>HMLEMIKSGKARAHTNIALIKYWGKKDEALIIPMNNSISVTLEKFYTETKVTFNDQLTQDQFWLNGEKVSGKELEKISKYMDIVRNRAGIDWYAEIESDNFVPTAAGLA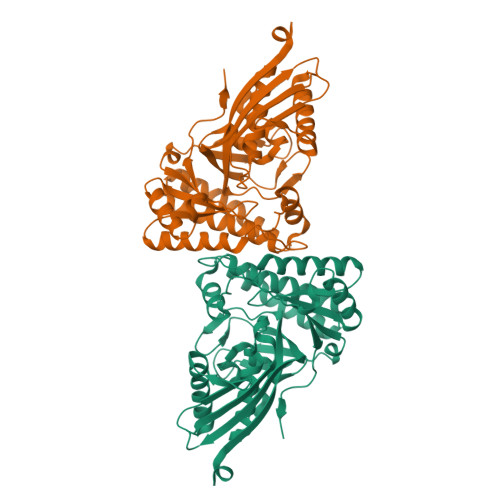SSASAYAALAAACNQALDMQLSDKDLSRLARIGSGSASRSIYGGFAEWEKGYSDETSYAVPLESNHFEDDLAMIFVVINQHSKKVPSRYGMSLTRNTSRFYQYWLDHIDEDLAEAKAAIQDKDFKRLGEVIEENGLRMHATNLGSTPPFTYLVQESYDVMALVHECREAGYPCYFTMDAGPNVKILVEKKNKQQIIDKLLTQFDNNQIIDSDIIATGIEIIE[2x]(2R)-2-hydroxy-3-oxobutyl dihydrogen phosphate | C4 H9 O6 P | 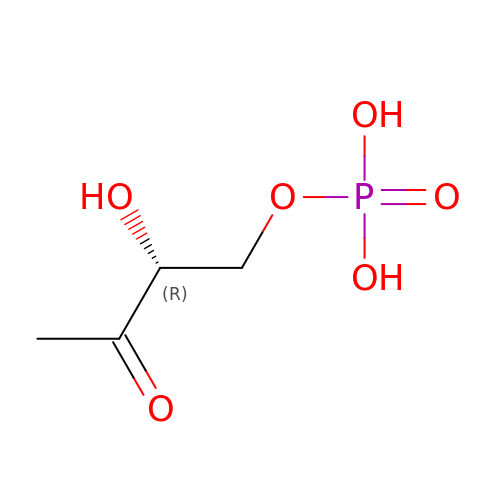OKYHYXLCTGGOLM-SCSAIBSYSA-N>[2x]STGNFDLFVVGSGFFGLTIAERAATQLGKRVLVIERRPHIGGNAYSEPEPETGIEVHKYGAHLFHTSNKRVWDYVRQFTDFTGYQHRVFAMHNGQAYQFPMGLGLVSQFFGRYFSPDEARALIAEQASEIDTKDAKNFEEKA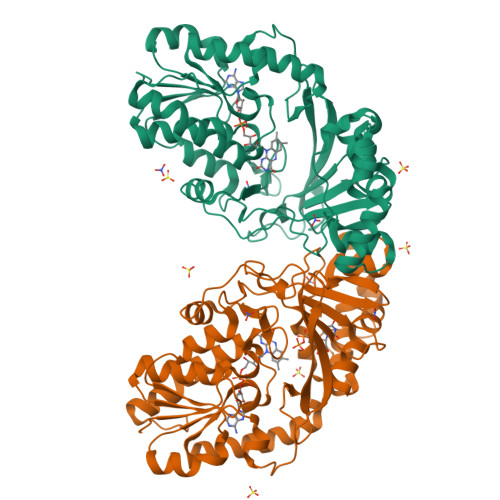ISLVGRPLYEAFIKHYTAKQWQTDPKDLPASNITRLPVRYTFDNRYFNDTYEGLPVEGYTKWLENMAADERIEVRLDTDWFDVRDDLRAANPDAPVVYTGPLDRYFDYAEGRLGWRTLDFELEVLETGDFQGTPVMNYNDLDVPYTRIHEFRHFHPERTYPTDKTVIMREYSRFADNDDEPYYPINTEADRAVLAAYRARAKAETASAKVLFGGRLGTYQYLDMHMAIASALSMFDNVLAPHLSEGASLVTEDESSKA>NEDICFIAGIGDTNGYGWGIAKELSKRNVKIIFGIWPPVYNIFMKNYKNGKFDNDMIIDKDKKMNILDMLPFDASFDTANDIDEETKNNKRYNMLQNYTIEDVANLIHQKYGKINMLVHSLANAKEVQKDLLNTSRKGYLDALSKSSYSLISLCKYFVNIMKPQSSIISLTYHASQKVVPGYGGGMS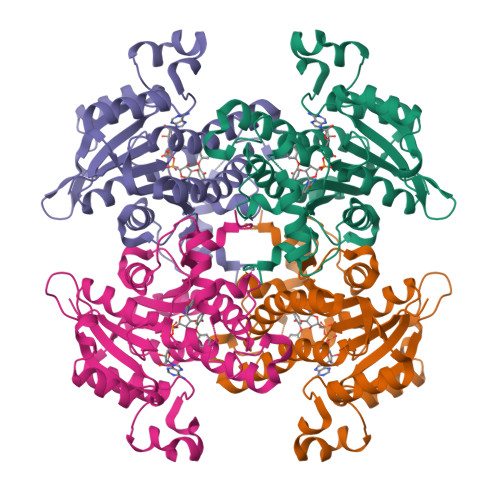SAKAALESDTRVLAYHLGRNYNIRINTISAGPLKSRAATAINKLNNTYENNTNQNKNRNRHDVHNIMNNSGEKEEKKISASQNYTFIDYAIEYSEKYAPLRQKLLSTDIGSVASFLLSRESRAITGQTIYVDNGLNIMFLPD[2x]>[6x]AWSHPQFEKTPATQPLINAEPAVAAQTEQNPQVGQVMPGVQGADAPVVAQNGPSRDVKLTFAQIAPPPGSMVLRGINPNGSIEFGMRSDEVVTKAMLNLEYTPSPSLLPVQSQLKVYLNDELMGVLPVTKEQLGKKTLAQMPINPLFISDFNRVRLEFVGHYQDVCEKPASTTLWLDVGRSSGLDLTYQTLNVKNDLSHFPVPFFDPSDNRTNTLPMVFAGAPDVGLQQASAIVASWFGSRSGWRGQNFPVLYNQLPDRNAIVFATNDKRPDFLRDHPAVKAPVIEMINHPQNPYVKLLVVFGRDDKDLLQAAKGIAQGNILFRGESVVVNEVKPLLPRKPYDAPNWVRTDRPVTFGELKTYEEQLQSSGLEPAAINVSLNLPPDLYLMRSTGIDMDINYRYTMPPVKDSSRMDISLNNQFLQSFNLSSKQEANRLLLRIPVLQGLLDGKTDVSIPALKLGATNQLRFDFEYMNPMPGGSVDNCITFQPVQNHVVIGDDSTIDFSKYYHFIPMPDLRAFANAGFPFSRMADLSQTITVMPKAPNEAQMETLLNTVGFIGAQTGFPAINLTVTDDGSTIQG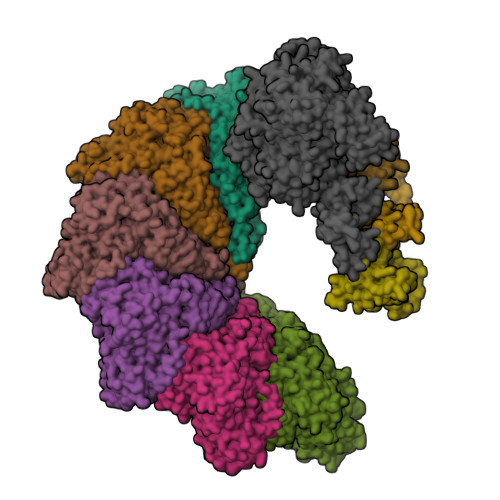KDADIMIIGGIPDKLKDDKQIDLLVQATESWVKTPMRQTPFPGIVPDESDRAAETRSTLTSSGAMAAVIGFQSPYNDQRSVIALLADSPRGYEMLNDAVNDSGKRATMFGSVAVIRESGINSLRVGDVYYVGHLPWFERVWYALANHPILLAVLAAISVILLAWVLWRLLRIISRRRLNPDNE;>MTQFTQNTAMPSSLWQYWRGLSGWNFYFLVKFGLLWAGYLNFHPLLNLVFAAFLLMPLPRYSLHRLRHWIALPIGFALFWHDTWLPGPESIMSQGSQVAGFSTDYLIDLVTRFINWQMIGAIFVLLVAWLFLSQWIRITVFVVAILLWLNVLTLAGPSFSLWPAGQPTTTVTTTGGNAAATVAATGGAPVVGDMPAQTAPPTTANLNAWLNNFYNAEAKRKSTFPSSLPADAQPFELLVINICSLSWSDIEAAGLMSHPLWSHFDIEFKNFNSATSYSGPAAIRLLRASCGQTSHTNLYQPANNDCYLFDNLSKLGFTQHLMMGHNGQFGGFLKEVRENGGMQSELMDQTNLPVILLGFDGSPVYDDTAVLNRWLDVTEKDKNSRSATFYNTLPLHDGNHYPGVSKTADYKARAQKFFDELDAFFTELEKSGRKVMVVVVPEHGGALKGDRMQVSGLRDIPSPSITDVPVGVKFFGMKAPHQGAPIVIEQPSSFLAISDLVVRVLDGKIFTEDNVDWKKLTSGLPQTAPVSENSNAVVIQYQDKPYVRLNGGDWVPYPQDYKDDDDK[3x];> MGSILTRWLLIPPVNARLIGRYRDYRRHGASAFSATLGCFWMILAWIFIPLEHPRWQRIRAEHKNLYPHINASRPRPLDPVRYLIQTCWLLIGASRKETPKPRRRAFSGLQNIRGRYHQWMNELPERVSHKTQHLDEKKELGHLSAGARRLILGIIVTFSLILALICVTQPFNPLAQFIFLMLLWGVALIVRRMPGRFSALMLIVLSLTVSCRYIWWRYTSTLNWDDPVSLVCGLILLFAETYAWIVLVLGYFQVVWPLNRQPVPLPKDMSLWPSVDIFVPTYNEDLNVVKNTIYASLGIDWPKDKLNIWILDDGGREEFRQFAQNVGVKYIARTTHEHAKAGNINNALKYAKGEFVSIFDCDHVPTRSFLQMTMGWFLKEKQLAMMQTPHHFFSPDPFERNLGRFRKTPNEGTLFYGLVQDGNDMWDATFFCGSCAVIRRKPLDEIGGIAVETVTEDAHTSLRLHRRGYTSAYMRIPQAAGLATESLSAHIGQRIRWARGMVQIFRLDNPLTGKGLKFAQRLCYVNAMFHFLSGIPRLIFLTAPLAFLLLHAYIIYAPALMIALFVLPHMIHASLTNSKIQGKYRHSFWSEIYETVLAWYIAPPTLVALINPHKGKFNVTAKGGLVEEEYVDWVISRPYIFLVLLNLVGVAVGIWRYFYGPPTEMLTVVVSMVWVFYNLIVLGGAVAVSVESKQVRRSHRVEMTMPAAIAREDGHLFSCTVQDFSDGGLGIKINGQAQILEGQKVNLLLKRGQQEYVFPTQVARVMGNEVGLKLMPLTTQQHIDFVQCTFARADTWALWQDSYPEDKPLESLLDILKLGFRGYRHLAEFAPSSVKGIFRVLTSLVSWVVSFIPRRPERSETAQPSDQALAQQHHHHHHLEHHHHHH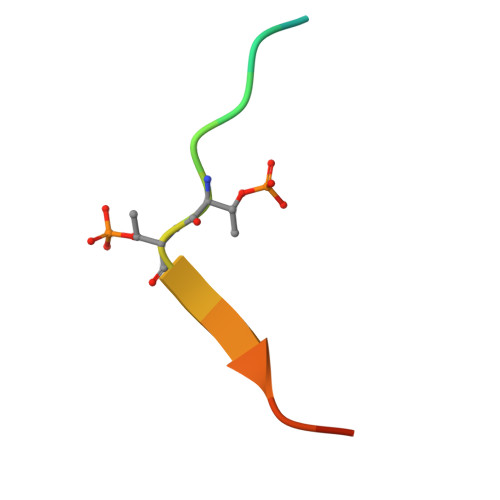> THPEWSFTTVRKKPDP> TPYDPLTLWTTPDPPPNCSLIQELDAKLTLCLTKNG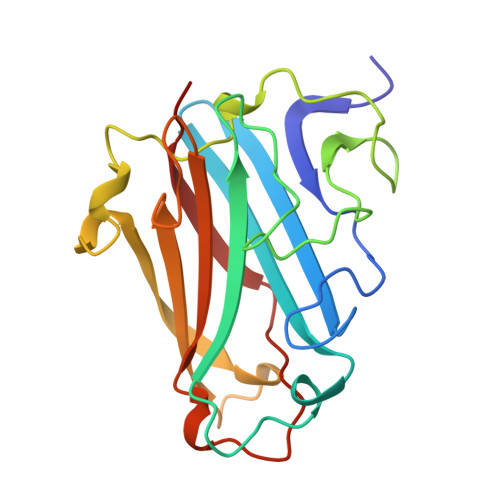SIVNGIVSLVGVKGNLLNIQSTTTTVGVHLVFDEQGRLITSTPTALVPQASWGYRQGQSVSTNTVTNGLGFMPNVSAYPRPNASEAKSQMVSLTYLQGDTSKPITMKVAFNGITSLNGYSLTFMWSGLSNYINQPFSTPSCSFSYITQE> MPTNFTVVPVEARADGAGDEAAERTEEPESPESVDQTSPTPGDGNPRENSPFINNVEVERESYF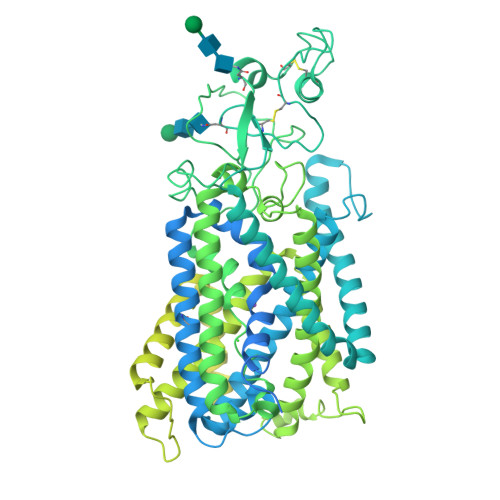EGKNMALFEEEMDSNPMVSSLLNKLANYTNLSQGVVEHEEDEDSRRREVKAPRMGTFIGVYLPCLQNILGVILFLRLTWIVGAAGVMESFLIVAMCCTCTMLTAISMSAIATNGVVPAGGSYYMISRSLGPEFGGAVGLCFYLGTTFAGAMYILGTIEIFLTYISPSAAIFQAETADGEAAALLNNMRVYGSCALALMAVVVFVGVKYVNKLALVFLACVVLSILAIYAGVIKTAFAPPDIPVCLLGNRTLANRNFDTCAKMQVVSNGTVTTALWRLFCNGSSLGATCDEYFAQNNVTEIQGIPGVASGVFLDNLWSTYSDKGAFVEKKGVSSVPVSEESRPGGLPYVLTDIMTYFTMLVGIYFPSVTGIMAGSNRSGDLKDAQKSIPTGTILAIVTTSFIYLSCIVLFGACIEGVVLRDKFGEALQGNLVIGMLAWPSPWVIVIGSFFSTCGAGLQSLTGAPRLLQAIARDGIIPFLQVFGHGKANGEPTWALLLTALICETGILIASLDSVAPILSMFFLMCYMFVNLACAVQTLLRTPNWRPRFKFYHWTLSFLGMSLCLALMFICSWYYALFAMLIAGCIYKYIEYRGAEKEWGDGIRGLSLNAARYALLRVEHGPPHTKNWRPQVLVMLNLDSEQCVKHPRLLSFTSQLKAGKGLTIVGSVLEGTYLDKHVEAQRAEENIRSLMSAEKTKGFCQLVVSSNLRDGASHLIQSAGLGGMKHNTVLMAWPEAWKEADNPFSWKNFVDTVRDTTAAHQALLVAKNIDLFPQNQERFSDGNIDVWWIVHDGGMLMLLPFLLRQHKVWRKCRMRIFTVAQVDDNSIQMKKDLQMFLYHLRISAEVEVVEMVENDISAFTYEKTLMMEQRSQMLKQMQLSKNEREREAQLIHDRNTASHTTATARTQAPPTPDKVQMTWTKEKLIAEKHRNKDTGPSGFKDLFSLKPDQSNVRRMHTAVKLNGVVLNKSQDAQLVLLNMPGPPKSRQGDENYMEFLEVLTEGLNRVLLVRGGGREVITIYSSNSLEVLFQ>GMILKTNLFGHTYQFKSITDVLAKANEEKSGDRLAGVAAESAEERVAAKVVLSKMTLGDLRNNPVVPYETDEVTRIIQDQVNDRIHDSIKNWTVEELREWILDHKTTDADIKRVARGLTSEIIAAVTKLMSNLDLIYGAKKIRVIAHANTTIGLPGTFSAR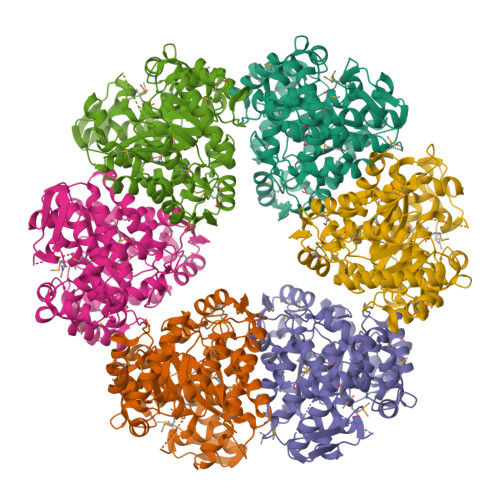LQPNHPTDDPDGILASLMEGLTYGIGDAVIGLNPVDDSTDSVVRLLNKFEEFRSKWDVPTQTCVLAHVKTQMEAMRRGAPTGLVFQSIAGSEKGNTAFGFDGATIEEARQLALQSGAATGPNVMYFETGQGSELSSDAHFGVDQVTMEARCYGFAKKFDPFLVNTVVGFIGPEYLYDSKQVIRAGLEDHFMGKLTGISMGCDVCYTNHMKADQNDVENLSVLLTAAGCNFIMGIPHGDDVMLNYQTTGYHETATLRELFGLKPIKEFDQWMEKMGFSENGKLTSRAGDASIFLK[6x]>QQLSDDEKLVAAFVKAVAYMSPRKIGALV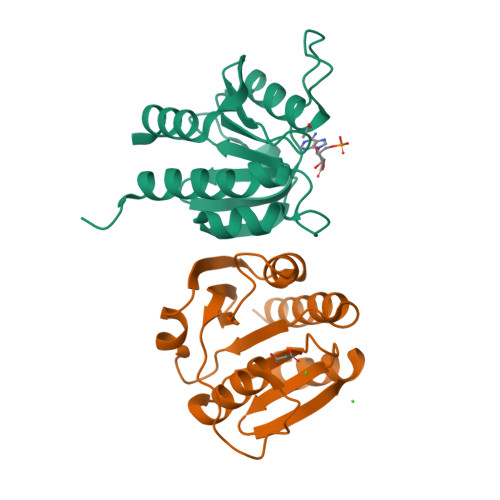SIEETQTLREYIATGIPLDADISGELLINIFIPNTPLHDGAVIVEGNKIAVSCAYLPLSESSHISKEFGTRHRAAIGLSEASDAFTFVVSEETGAISVAYKGDFIHDLSLEAFEVLLREHFI[2x]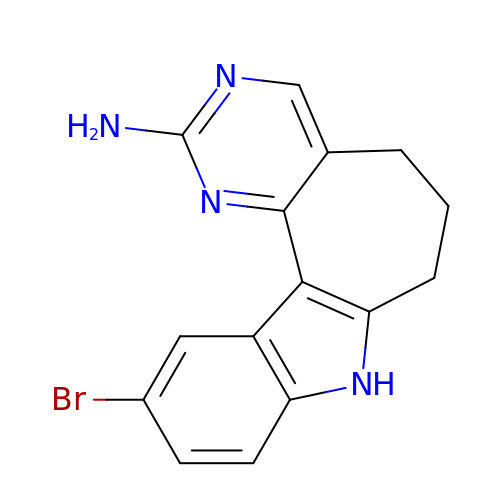11-bromo-5,6,7,8-tetrahydropyrimido[4',5':3,4]cyclohepta[1,2-b]indol-2-amine | C15 H13 Br N4 | MEOWHQIIZUZBTO-UHFFFAOYSA-N FtsEX is a membrane complex widely conserved across diverse bacterial genera and involved in critical processes such as recruitment of division proteins and in spatial and temporal regulation of muralytic activity during cell division or sporulation. The component FtsX is an integral membrane protein, whereas FtsE is an ATPase and is required for the transmission of a conformational signal from the cytosol through the membrane to regulate the activity of cell wall hydrolases in the periplasm. Here, we provide the first three-dimensional (3D) structure of FtsE from the notorious pathogen S. pneumoniae, and we show that it presents all the conserved structural motifs of the NBD members of the ABC transporter family. The nucleotide-binding site is located in lobe I near the interface between the two lobes and presents the nucleotide sandwiched between the Walker A and B motifs.

Two different crystal forms in complex with ADP were obtained in the same crystallization conditions belonging to two different space groups, P 1 and P 21. P 1 crystals contain one molecule per asymmetric unit and diffract up to 1.36 Å resolution, while P 21 crystals contain three molecules per asymmetric unit and diffract up to 1.57 Å resolution. Unless otherwise indicated, the description of the monomer structure provided here is for the highest-resolution crystal form belonging to space group P 1. FtsE binds ADP by both van der Waals and polar interactions. The Walker A (P-loop) motif wraps over the β-phosphate of ADP forming an extensive hydrogen bond network with main-chain nitrogen atoms of G40 to K43. The position of the K43 side chain, essential for nucleotide binding through interaction with the β-phosphate, is stabilized by H bonds with main-chain oxygen atoms of G37 and P38. The switch histidine (H197) that stabilizes the transition-state geometry in the ADP-bound state interacts with the β-phosphate through two interspersed water molecules. The A-loop provides an aromatic side chain (Y13) that packs against the purine ring of adenine involving a π-stacking interaction and positions the base and ribose of the nucleotide. This interaction provides an additional binding free energy for ADP through an extensive hydrophobic interaction that buries 48.4 Å2 of surface area (calculated with PDBePISA v1.52) between its aromatic ring and the adenine base of ADP. Superposition of the NBD of MacB with the FtsE-ADP complex results in an excellent fit with an RMSD value of 1.0 Å for 174 Cα atoms.

> MSIIEMRDVVKKYDNGTTALRGVSVSVQPGEFAYIVGPSGAGKSTFIRSLYREVKIDKGSLSVAGFNLVKIKKKDVPLLRRSVGVVFQDYKLLPKKTVYENIAYAMEVIGENRRNIKRRVMEVLDLVGLKHKVRSFPNELSGGEQQRIAIARAIVNNPKVLIADEPTGNLDPDNSWEIMNLLERINLQGTTILMATHNSQIVNTLRHRVIAIENGRVVRDESKGEYGYDD One major group, the Bacilladnaviridae family of single-stranded DNA viruses, infects diatoms in marine environments. The icosahedral capsid of bacilladnaviruses is formed by T = 3 asymmetrical units, in contrast to the smaller T = 1 capsids found in other Cressdnaviricota groups, presumably reflecting the need to package larger genomes. The bacilladnavirus CP contains the common viral jelly-roll fold that forms the bulk of the capsid and an additionalß-sheet projection domain. In contrast, the CPs are highly variable and thought to have been acquired from different RNA viruses through multiple independent horizontal gene transfer (HGT) events.

The structure of the ClorDNAV capsid was determined using single-particle cryo-EM with imposed icosahedral symmetry. The final reconstruction reached a resolution of 2.2 Å, with local resolutions ranging from 1.82 to 35 Å. The ClorDNAV capsid has T = 3 symmetry and consists of 180 CP protomers. The asymmetric unit contains three quasi-equivalent CP subunits, designated A, B, and C, following the nomenclature previously established for CtenDNAV-II. We were able to model residues 46/47 to 388 of the 390-residue CP. The three CP subunits are nearly identical and adopt a canonical jelly-roll fold composed of eight β-strands arranged into two antiparallel β-sheets (BIDG and CHEF). In addition to the canonical strands, the structure includes additional ß-strands in each sheet (I’BIDGG’I’’ and C’’C’CHEF). A third β-sheet, composed of seven antiparallel strands formed by loop extensions between strands C-D (2x), E-F (2x), and G-H (3x), creates a surface-exposed projection domain. In contrast, in ClorDNAV, all C-termini are oriented toward the capsid interior, similar to subunit C of CtenDNAV-II. As a result, ClorDNAV contains two interior-facing helices per subunit, whereas CtenDNAV-II contains only one, and only from subunit C. In ClorDNAV, no such density was observed, and positively charged arginine, lysine, or histidine residues within the interface region either face outward (e.g., R80 of ClorDNAV) or are positioned much further apart than in CtenDNAV-II.

>MAGRRKQRRSRAPRRKRTTGRKTLKRKADSRATPAKSTRKRTKTVSGAAKHHAVRVKPFSNATTQPKIPDGLLTSSLSRRLQNVVGVRNGNSPSVHAGSDVMHVVIAPTLGVPVMIANSAEGVLKRPGLSQESSFIGFPGQTVGFENLIESTGVPTWPPTIPTGQKLENKGGFVLWRIISQGLRIDLANSDEENDGWFEACRFNWRNVPRDVCMTPLDGSTTTNSIGIAPNPLWLEEVGYGMAMVEQPGYKSGLLKDIKKAEFMLHPRTTTHDPTLIDPFEYGGSMTSSGGIDNVYYPSDNVSGNAVRFRDMGVDQNMDWIYIRLHCRPNNGTSSLGSNFLFNVIQNVEVAFNPSSDFAAFQTINKADTKTKMVADGLNNNPDVFNGRRK[3x]>SMATSNPTVVDIHTHMYPPQYIKILESRTTIPLVRKFPQAPEPRLILLEAELGDLEKAINDPSAKPPGRPLTSHFASLDQKIHFMDTHRIDISVISLANPWLDFVHASHAGDIAESVNDEFSDMCGKHHGRLFFFGTLPLTAPLETLLASISHLAALKYCRGVILGTSGLGKGLDDPHLIPIFEALAAANLTIFLHPHYGLPNDVWGPRAGEYGHVLPLALGFPMETTIAVARMYLAGVFDQVRDLRMVLAHSGGT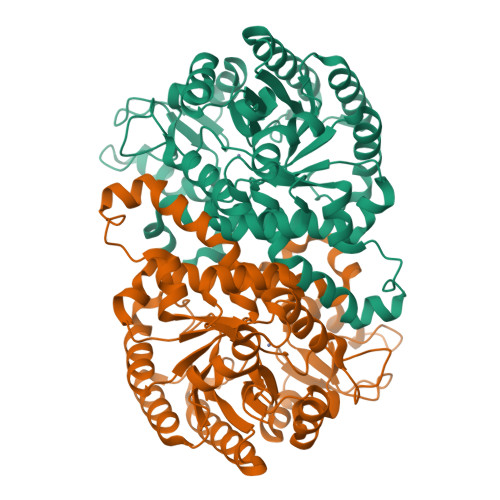LPFLAGRIESCIFHDGQLVRQGKVGENRRTVWDVLKEQVYLDAVIYSEVGLKAAIDASGSDRLMFGTDHPFFPPITTDEQGQWESVSLNAQAVAEAVGEGSAEARAIMGSNAIRVLRLEEKA[3x]>[4x]GGGGSMADPEVVVS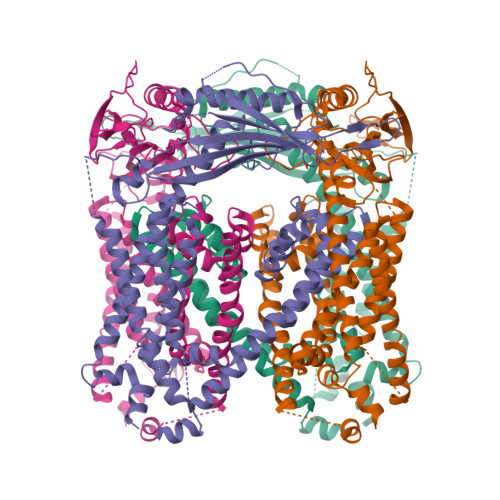SCSSHEEENRCNFNQQTSPSEELLLEDQMRRKLKFFFMNPCEKFWARGRKPWKLAIQILKIAMVTIQLVLFGLSNQMVVAFKEENTIAFKHLFLKGYMDRMDDTYAVYTQSDVYDQLIFAVNQYLQLYNVSVGNHAYENKGTKQSAMAICQHFYKRGNIYPGNDTFDIDPEIETECFFVEPDEPFHIGTPAENKLNLTLDFHRLLTVELQFKLKAINLQTVRHQELPDCYDFTLTITFDNKAHSGRIKISLDNDISIRECKDWHVSGSIQKNTHYMMIFDAFVILTCLVSLILCIRSVIRGLQLQQEFVNFFLLHYKKEVSVSDQMEFVNGWYIMIIISDILTIIGSILKMEIQAKSLTSYDVCSILLGTSTMLVWLGVIRYLGFFAKYNLLILTLQAALPNVIRFCCCAAMIYLGYCFCGWIVLGPYHDKFRSLNMVSECLFSLINGDDMFATFAKMQQKSYLVWLFSRIYLYSFISLFIYMILSLFIALITDTYETIKQYQQDGFPETELRTFISECKDLPNSGKYRLEDDPPVSLFCCCKK>METDNVELAQSKRKVVLAEQGSFYIGGRTVTGPGKFDPSKPVIPYSNEGATFYINQMYVNFQAPVRPRGLPLVFWHGGGLTGHIWESTPDGRPGFQTLFVQDRHTVYTIDQPGRGRGNIPTFNGPFGQLEEESIVNTVTGNSSKEGAWVRDRLGPAPGQFFENSQFPRGYEDNYFKEMGFSPSISSDEIVDAVVKLVTHIGPCVLVTHSASGVLGMRVATHAKNVRGIVAYEPATSIFPKGKVPEIPPLADKKSQIFPPFEIQESYFKKLAKIPIQFVFGDNIPKNPKSAYWFLDWWRVTRYAHSLSLEA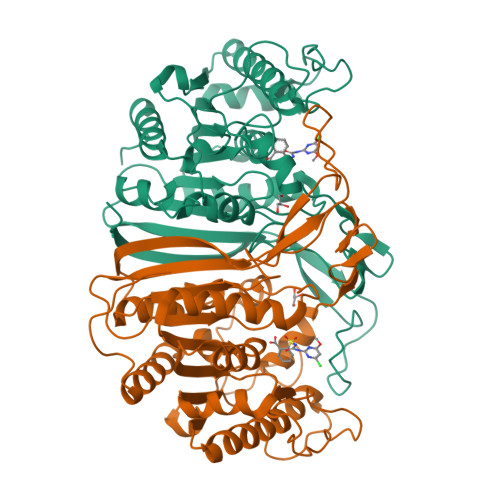INKLGGQASLLDLPTAGLRGNTHFPFTDRNNVQVASLLSDFLGKHGLDQNESLEHHHHHH[4x]> SGDYRVQNTSLEAIVQNASSDNQGIQLSAVQAARKLLSSDRNPPIDDLIKSGILPILVHCLERDDNPSLQFEAAWALTNIASGTSEQTQAVVQSNAVPLFLRLLHSPHQNVCEQAVWALGNIIGDGPQCRDYVISLGVVKPLLSFISPSIPITFLRNVTWVMVNLCRHKDPPPPMETIQEILPALCVLIHHTDVNILVDTVWALSYLTDAGNEQIQMVIDSGIVPHLVPLLSHQEVKVQTAALRAVGNIVTGTDEQTQVVLNCDALSHFPALLTHPKEKINKEAVWFLSNITAGNQQQVQAVIDANLVPMIIHLLDKGDFGTQKEAAWAISNLTISGRKDQVAYLIQQNVIPPFCNLLTVKDAQVVQVVLDGLSNILKMAEDEAETIGNLIEECGGLEKIEQLQNHENEDIYKLAYEIIDQFFSSDDIDEDPSLVPEAIQGGTFGFNSSANVPTEGFQF

Active transport of proteins from the cytoplasm to the nucleus is mediated by a family of nuclear transport receptors known as importins (or karyopherins), together with a number of ancillary proteins including nucleoporins and Ran1–3. Importin α is constructed from an N-terminal importin β-binding (IBB) domain and a C-terminal NLS binding domain featuring ten armadillo (ARM)-repeat motifs. The W proteins of henipaviruses share a common N-terminal domain with P and V proteins, but have a unique NLS bearing C-terminal domain that is recognised preferentially by importins α3 and α4 (KPNA4 and KPNA3), rather than the better characterised importin α1 (KPNA2). In this study, we present high-resolution structures of importin α isoform adaptors bound to the NLS regions of HeV W and NiV W, providing insights into the molecular basis of importin α isoform specificity.

To extend on the structural repertoire of importin α structures, we tested whether these ARM repeats are similar in the structures of importin α isoforms that do not contain bound cargo. Importin α1 and α3, crystallised in P212121 and P1211 space groups, respectively, both contained one chain in the ASU. This is the first report of these adaptors being crystallised without cargo bound in the NLS-binding pockets, although a dimer of importin α1 has been reported previously. Superposition of importin α3 in the cargo free and bound forms showed that the N-terminal ARM repeats 1–4 are repositioned by up to 5 Å, consistent with previous findings that a more flexible hinge region is present in importin α315. However, the position of ARM repeats 7 and 8 was retained in both the cargo free and bound forms of importin α3. These results suggest that ARMs 7 and 8 do not undergo conformational changes to accommodate binding of the W NLS in either importin α1 or α3. In addition, we show through structural comparisons between apo- and W bound-importin α3, that structural changes in the N terminus were not associated with direct binding interactions in this region. The study by Sankhala et al. 15 indicated that the NLS of RCC1 binds in the major binding site of ARMS 2–4 of both importin α1 and α3, with additional interactions occurring at the N terminus of importin α3 ARM repeats 1–4 and the β-propeller region of RCC1, mediated by flexibility and rotation of importin α3 in ARM repeats 1–2. This mechanism of isoform specificity is well suited to cargo containing NLSs at the N terminus, and our structural data of the unbound and NLS-bound forms of importin α3 supports this model.>[2x]MHIERLAVDESVGRAMPPQRFIEALSDLGVPVEFAGEDEQFGPGDAVASFGHRDAFLDADWVHCIRAGYDEFPVGVYEEAGTYLTNSTGIHGTTVGETVAGYMLTFARRLHAYRDAQHDHAWDLPRYEEPFTLAGERVCVVGLGTLGRGVVDRAAALGMEVVGVRRSGDPVDNVSTVYTPDRLHEAIADARFVVLATPLTDETEGMVAAPEFETMREDASLVNVARGPVVVESDLVAALDSGDIAGAALDVFSEEPLPEDSPLWDFEDVLITPHVSAATSKYHEDVAALIRENIEKIATGDELTNRVV

Here we describe the molecular basis of the reaction mechanism and dual NADH/NADPH-specificity of D2HDH, a 2-hydroxyacid dehydrogenase from the extreme halophile Haloferax mediterranei, an organism whose proteins have to remain active in high intracellular concentrations of KCl. Sequence analysis has identified D2HDH as a member of the DDH clade of the D-isomer specific 2-hydroxyacid dehydrogenase enzyme family (2HADH), which has potential applications in the synthesis of chiral fine chemicals including alcohols, and hydroxy or amino acids from ketones or ketoacids. Structural studies have shown that all members of this family share a common fold based on two domains, which cycle between open and closed conformational states that serve to close the inter-domain cleft, bringing the substrates together during catalysis. The D2HDH dimer has an overall ellipsoidal appearance in which each monomer is folded into two domains (d1; residues 1–92 and 283–308 and d2; residues 93–282).

Interestingly, the structures of the D2HDH complexes determined in this study have shown that, dependent upon the crystallisation conditions used, the 2-ketoacid substrate can be trapped in the crystal structure in two different orientations, representing a catalytic or abortive mode of binding. In both the productive and abortive modes of substrate binding the 2-ketohexanoic acid alkyl side chain occupies a similar position in the active site, but is twisted as a result of a 120° rotation to the C2-C3 torsion angle.trans-4-{(1R)-2-[(5S)-6-fluoro-5H-imidazo[5,1-a]isoindol-5-yl]-1-hydroxyethyl}cyclohexan-1-ol | C18 H21 F N2 O2 | 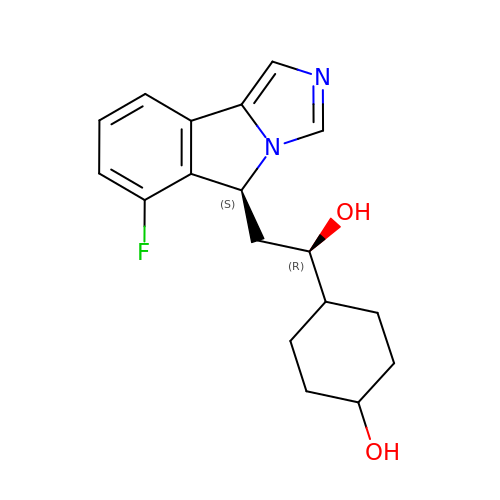YGACXVRLDHEXKY-WXRXAMBDSA-N> TYFITMNNARNFFIQQLESNAQDTATSLGLSLSQSLINHDVPTMDSMVKAVFDRGYFS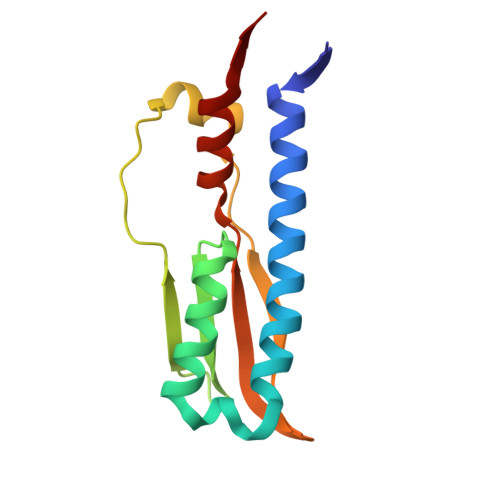SIKVQDIKGKVIILKKQLPQESDIPQWFVNLIKWPSTEKSSLIMDGWMQAGVVLVASDPSYVYASLWRNAVEM PLC enzymes catalyze the hydrolysis of inositol lipids, mainly phosphatidylinositol 4,5-bisphosphate (PIP2) to second messengers inositol 1,4,5-trisphosphate (IP3) and diacylglycerol. The catalytic activity in all PLCs is encapsulated within the TIM (triose-phosphate isomerase) barrel fold structure, which, in most isoforms, together with a PH domain, C2 domain, and EF hands, forms a common PLC core. PLCγ enzymes are characterized by an array of domains, referred to as “γ-specific array (γSA)” or as “regulatory region,” encompassing the sPH, nSH2, cSH2, and SH3 domains. Recent structural insights have revealed PLCγ1 in its autoinhibited state, which is characterized by an inhibitory interface between the catalytic PLC core domains and the regulatory γSA.

The geometry of the active site is largely conserved compared to the structure of the related PLCδ1—coordination of phosphate 1 of IP3 involves H335, H380, and Ca2+, the position 4 and 5 phosphates engage in electrostatic interactions, including interaction of the position 4 phosphate with K462 and R1010, and the 2-hydroxyl group is ligated to Ca2+ (12). Despite the presence of excess IP3 in the crystallization buffer, IP3 binding to the nPH domain was not observed. This suggests that unlike PLCδ1, the nPH of PLCγ1 lacks a canonical PIP2 binding site. Similarly, Ca2+ binding to the C2 domain was not observed. First, there are hydrophobic, electrostatic, and hydrogen bonded contacts between the sPH and the TIM barrel, centered on the hydrophobic ridge near the entrance to the active site. A second interface is formed between the C2 and cSH2 domains. M1166 and F1167, which form the hydrophobic tip of a loop on the C2 domain, bury into a hydrophobic pocket formed by F706, L746, and Y747 on the cSH2 domain. There is additionally a weak interaction between the EF-hand and nSH2 domains, stabilized by a single hydrogen bond between K175 and T576, which is positioned slightly differently from the previous structure. The PLCγ1 nPH is more akin to the ArhGAP9 PH domain, which points clusters of basic residues outward toward the membrane, and has a noncanonical PIP binding pocket between the β1-β2 and β5-β6 loops. This analysis reconciles our findings that the nPH is critical for liposome binding and catalytic activity and yet has no IP3 binding site detected in the crystal structure. The PIP2 headgroup observed in the simulations, however, is not as deep in the active site as observed for IP3 in the structure.

> SQAEVLHLCRSLEVGTVMTLFYSKKSQRPERKTFQVKLETRQITWSRGADKIEGSIDIREIKEIRPGKTSRDFDRYQEDPAFRPDQSHCFVILYGMEFRLKTLSLQATSEDEVNMWIKGLTWLMEDTLQAATPLQIERWLRKQFYSVDRNREDRISAKDLKNMLSQVNYRVPNMRFLRERLTDFEQRSGDITYGQFAQLYRSLMYSAQKTMDLPFLETNTLRTGERPELCQVSLSEFQQFLLEYQGELWAVDRLQVQEFMLSFLRDPLREIEEPYFFLDELVTFLFSKENSVWNSQLDAVCPETMNNPLSHYWISSSHNTYLTGDQFSSESSLEAYARCLRMGCRCIELDCWDGPDGMPVIYHGHTLTTKIKFSDVLHTIKEHAFVASEYPVILSIEDHCSIAQQRNMAQHFRKVLGDTLLTKPVDIAADGLPSPNQLKRKILIKHKKLAEGSAYEEVPTSVMYSENDISNSIKNGILYLEDPVNHEWYPHYFVLTSSKIYYSEETSSDQGNEDEEEPKEASGSTELHSSEKWFHGKLGAGRDGRHIAERLLTEYCIETGAPDGSFLVRESETFVGDYTLSFWRNGKVQHCRIHSRQDAGTPKFFLTDNLVFDSLYDLITHYQQVPLRCNEFEMRLSEPVPQTNAHESKEWYHASLTRAQAEHMLMRVPRDGAFLVRKRNEPNSYAISFRAEGKIKHCRVQQEGQTVMLGNSEFDSLVDLISYYEKHPLYRKMKLRYPINEEALEKIGSGSTFKCAVKALFDYKAQREDELTFTKSAIIQNVEKQDGGWWRGDYGGKKQLWFPSNYVEEMINPAILEPEREHLDENSPLGDLLRGVLDVPACQIAIRPEGKNNRLFVFSISMPSVAQWSLDVAADSQEELQDWVKKIREVAQTADARLTEGKMMERRKKIALELSELVVYCRPVPFDEEKIGTERACYRDMSSFPETKAEKYVNKAKGKKFLQYNRLQLSRIYPKGQRLDSSNYDPLPMWICGSQLVALNFQTPDKPMQMNQALFMAGGHCGYVLQPSTMRDEAFDPFDKSSLRGLEPCVICIEVLGARHLPKNGRGIVCPFVEIEVAGAEYDSTKQKTEFVVDNGLNPVWPAKPFHFQISNPEFAFLRFVVYEEDMFSDQNFLAQATFPVKGLKTGYRAVPLKNNYSEDLELASLLIKIDIFPAK>[2x]MPITWMRMRPWLEMQINSNQIPGLIWINK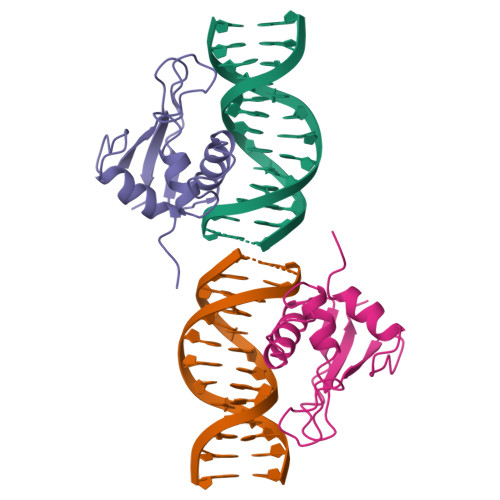EEMIFQIPWKHAAKHGWDINKDACLFRSWAIHTGRYKAGEKEPDPKTWKANFRCAMNSLPDIEEVKDQSRNKGSSAVRVYRMLP O-TOLUENESULFONAMIDE | C7 H9 N O2 S | 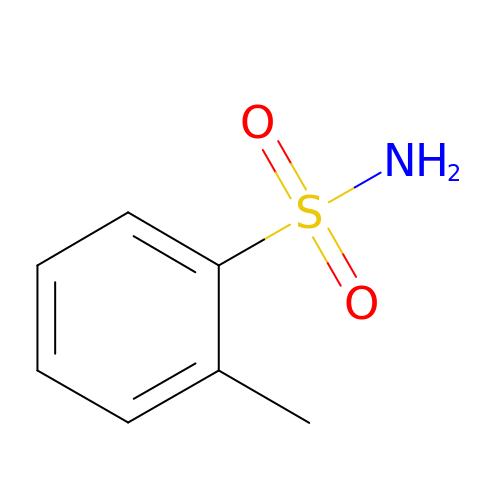YCMLQMDWSXFTIF-UHFFFAOYSA-N>MSQKEVYDAAGFGNPVSRGVHPAIIVVDFSYGFTDLQYPTASDASLQMSRTKEICDLARALEFPVIFTTIAYHPGEIPMLPWLEKSSGMAALLYGSRLVEIDMATGIQPNDVVVVKKGASSFFGSTLSS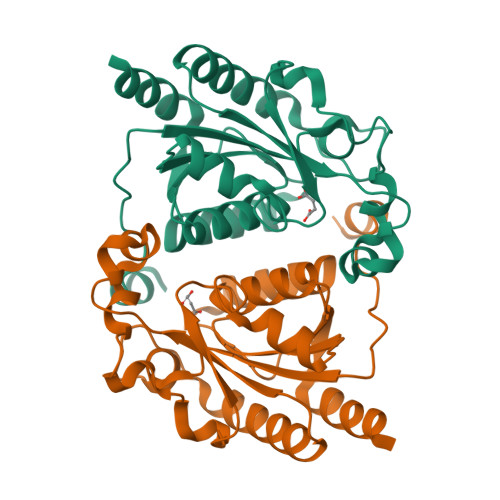LLAGTNTDTVVVTGATTSGAVRATVVDAVQSGFKVLVPADCCADRAKGPHEASLYDIQQKYGDVTDSDDILKWLRSVAG[8x]>[2x]MSTKVKKTTQLKQMLNSK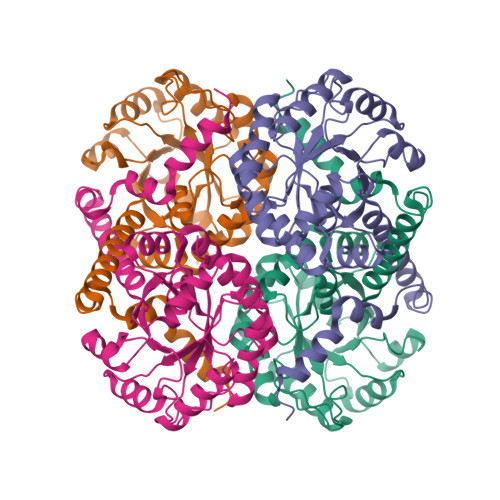DLEFIMEAHNGLSARIVQEAGFKGIWGSGLSVSAQLGVRDSNEASWTQVVEVLEFMSDASDVPILLDADTGYGNFNNARRLVRKLEDRGVAGACLEDKLFPKTNSLHDGRAQPLADIEEFALKIKACKDSQTDPDFCIVARVEAFIAGWGLDEALKRAEAYRNAGADAILMHSKKADPSDIEAFMKAWNNQGPVVIVPTKYYKTPTDHFRDMGVSMVIWANHNLRASVSAIQQTTKQIYDDQSLVNVEDKIVSVKEIFRLQRDDELVQAEDKYLPKN>MGGEVEEPEPQMVLSPLTSAAIFLVVTIDSGGEDTVRDLLSDVASLERAVGFRAQPDGRLSCVTGIGSEAWDRLFSGARPAGLHPFRELDGPVHRAVATPGDLLFHIRASRLDLCFALATEIMGRLRGAVTPQDEVHGFKYFDERDMLGFVDGTENPTGAAARRAVLVGAEDPAFAGGSYAVVQKYLHDIDAWEGLSVEAQERVIGRRKMTDVELSDDVKPADSHVALTSVTGPDGSDLEILRDAMPFGSVGREEFGTYFIGYARTPEVTETMLERMFLGTASAPHDRILDFSTAVTGSLFFTPAADFLEDLSARP[6x]

Using an X-ray free electron laser (XFEL), we have previously determined room-temperature (RT) serial femtosecond crystallography (SFX) structures of the ferric and Compound I redox states of DtpB,26 a B-type member of the dye-decolorizing peroxidase (DyP) family. Such an approach results in “pristine” DtpB structures that do not exhibit the effects of X-ray-generated radiation damage. The RT-SFX DtpB ferric and Compound I structures revealed that the distal heme pocket, which is composed of an Asp–Arg–Asn triad, was void of H2O molecules. DtpB, therefore, represents an exemplar of a His–heme-ligated peroxidase in which the distal heme pocket favors a dry site. By disrupting the distal heme pocket Asp–Asn–Arg triad in DtpB, our RT-SFX structures reveal that a wet site can be formed.

To assess whether disruption of the Asp–Arg–Asn triad in DtpB leads to a wet distal heme pocket, microcrystals of each variant in the Fe(III)–heme state were produced and subjected to RT-SFX crystallography using a high viscosity extruder sample delivery system at the SACLA XFEL beamline BL2 EH3. For all variants, well-defined electron density peaks were present in the distal heme pocket, consistent with the presence of resident H2O molecules. In the N245A variant, only one resident H2O is found, and in the R243A variant, four resident H2O molecules are observed, with three of these accommodated within the distal pocket and the fourth positioned in the space vacated by the Arg243 side chain. In the N245A variant, the single H-bonded distal pocket H2O molecule occupies the space left by the amino group of the Asn245 side chain but is positioned too far from Fe(III)–heme to initiate a bonding interaction. Thus, Fe(III)–heme in the N245A variant remains pentacoordinate, as in WT DtpB. Notably, the H-bonded Asp–H2O does not have the same spatial stereochemistry as found for the Asp–H2O unit in DtpA (an A-type DyP possessing a wet distal heme pocket that uses the Asp–H2O unit to facilitate Compound I formation). Thus, the Asp–H2O arrangement in the N245A variant would not be expected to facilitate proton movement in Compound I formation. The N245A variant can be considered to have a “semi-dry” pocket, in which case, the effect of pKa on Fe(III)–H2O2 would be less and is evident inFigure 2, with the pKa only partially visualized above pH 4.5. The pH dependence of the N245A variant is closer to that of WT, but the data provide evidence of an acidic pKa of < 4. Thus, the D152A and D152A/N245A variants (fully wet) are almost fully populated at 76 and 93%, respectively, while the “semi-dry” N245A variant is 52% populated.>MKNLRYKLLLFVFIGFWGLLALNLFILSVKNQEYYEKLAERNMTKKEFLVPTRGNITDRNDEFLATNELVFGVFLPSGLKQKDLLEKIEIIQKFFPNFSKETLLNNYQKENSLYNHNLIKVVGFIPYATMQPLYAKLIQTQGIFALPLDKRYYPNNALASHVLGYVGVASLQDLKDDEENQYSQIVGKTGIEKEYNKLLQGKVGYKIMRVNALNQELATLEVVLPSTNNHLQLSLDKRLQKEADKLFENKRGAILVMDAENGELLVAGSYPEYNLNDFVGGISQDKWQKLQDDIYNPLLNRFANALYPPGSVVKMGVGLSFLENLHITENTTIPTPPFIEVGKHKFRDWKKTGHGNSNLYKAIRESVDVYFYKFGLEISIEKLSKTLREVGFGEKTGVDLPNEFVGIVPDNLWKLKRFNQDWRVGDTLITAIGQGSFLATPLQVLAYTGLIATGKLATPHFAINNKQPLKDPLNSFQKKKLQALRVGMYEVCNHKDGTAYHSTRGSKITLACKTGTAQVVEIAQNIVNRMKEKDMEYFHRSHAWITAFLPYEKPKYAITILVEHGEGGSKLGGLLVKMSNKLYELGYLHHHHHH[2x];>[4x]MRFYFKFLWLLGIFLIFYFLDFKGSSSYISDRIKNALMNAKNSLLDNVQAYFFQAQNIKEFQKERLILEALKLENADLKERLNSIYPLENPKMTYTPTFMTSFISLEDTHSVSLNPIVNLEENKIYGLVSHNQAIGIAVLEKGRLNGF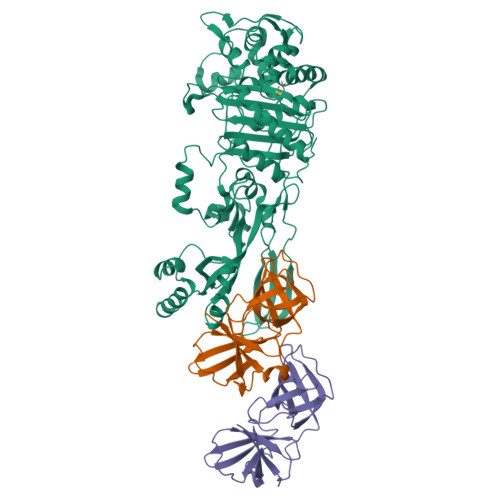LNAHKRCAYSVMIGQNQVLGFIGTNFKQELVVDFIVPSAEINIGDQVLTSGLDGIFGAGVFVGEVSSIEDHYTYKSAVLKNAFLSGAKLLRHVFLSDVKN N-{2-[(2Z)-3-chlorotetradec-2-enamido]ethyl}-N~3~-[(2R)-2-hydroxy-3,3-dimethyl-4-(phosphonooxy)butanoyl]-beta-alaninamide 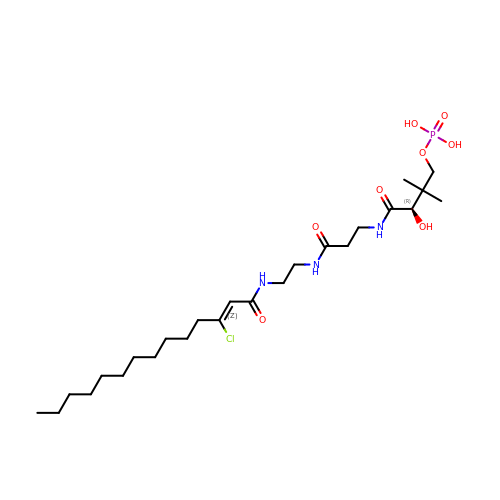| C25 H47 Cl N3 O8 P | AFBUYZJEABFPSA-LQAKIXKWSA-N>MINAQLLQSMVDASNDGIVVAEKEGDDTILIYVNAAFEYLTGYSRDEILYQDCRFLQGDDAASGATARIRKAMAEGRPCREVLRNYRKDGSAFWNELSITPVKSDFDQRTYFIGIQKDVSRQVELERELAELRARPKPDERA[2x]

By using a flavin transferase and carving a flavinylation motif in target proteins, we demonstrate that “dissociable” flavoproteins can be turned into covalent flavoproteins. Specifically, four different flavin mononucleotide-containing proteins were engineered to undergo covalent flavinylation: a light-oxygen-voltage domain protein, a mini singlet oxygen generator, a nitroreductase, and an old yellow enzyme-type ene reductase. The crystal structures of the designed covalent flavoproteins confirmed the designed threonyl-phosphate linkage. The elucidated crystal structures confirm that the covalent attachment does not significantly perturb the binding and microenvironment of the redox active part of the flavin cofactor.

The six preceding residues of the motif were subsequently chosen by established rational protein engineering considerations such as to minimize the structural change at a position, e.g., retaining a glycine at position 65 when compatible with the motif, mutating to an alanine whenever in doubt (e.g., D62A, not D62ILVF), and minimizing hydrophobic exposure at the surface (e.g., Q63S, not Q63T, which would introduce a water-exposed hydrophobic methyl group). This resulted in two PpSB1-LOV variants, each with six point mutations, which are further referred to as PpSB1-LOV-F1 (D60D + R61A + D62A + Q63S + L64G + G65A + R66T) and PpSB1-LOV-F2 (L64D + G65G + R66A + A67S + R68G + I69A + R70T). To gain insight into the structural consequences of the covalent tethering and the introduced mutations, we determined the crystal structure of PpSB1-LOV-F1. Residues 61–63 are in a loop, and residues 64–66 are part of an α-helix similar to other LOV domain proteins. The isoalloxazine and ribityl moieties of FMN have the same interactions with the protein side chains. The phosphate atom, however, has a different position, 1.9 Å away toward Thr66, to which it is covalently attached, by a changed angle of C4′–C5′–O5′. From the interactions with guanidino groups of Arg54, Arg61, Arg66, and Arg77 in wild-type PpSB1-LOV, only Arg54 and Arg70 are retained due to the mutations. Variant F1 displays the fastest dark recovery, accelerating from almost 1 day (1150 min) for wild-type PpSB1-LOV to about 5 min in the case of PpSB1-LOV-F1. Interestingly, PpSB1-LOV-F1 and -F2, both containing covalent FMN, exhibited a quantum yield 3.5 times and 2 times higher than that of the wild-type LOV protein, respectively. The effect was largest for PpSB1-LOV-F1, which displayed an apparent melting temperature (Tm) that was 10.5 °C higher when compared with that of the wild-type LOV protein.> MGIISYVKKLFKRPAGEIMRMSSGNIGVYKLDDSRVDYELARELYQNKNANYKLGSSFVRPIVNSTTGFMGVPHFQIEDEEAQYILDEFVLDNTSKMLKTHTDSLKQGDCYIWITREERENPLYPDKKVRLIYNFISPEEVKEIILDPTTKEPIAYILESQNEWTDLGENKRKAKVKQIITAESRFVEVEGDKIEGLEEGETPNVWGFIPIIHFKNEADETLKYGQSDIEPIEPLLKAYHDVMLHALKGSKMHSTPKLKLKLTDVASFLAHNFGVEDPVKFAKEGGKINLDGHEILFLNKDEEAEFVEVKSAIGDAKELLKLLFYCIVDVSETPEFIFG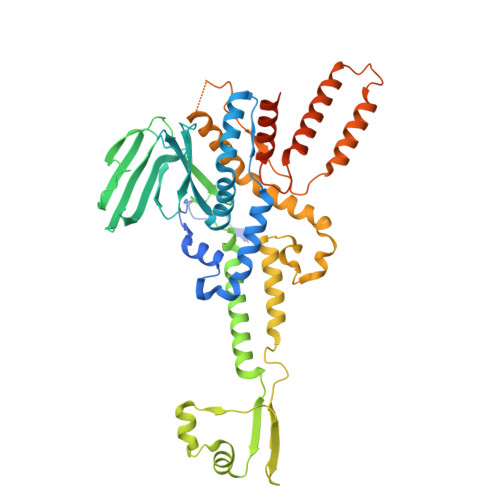VHTPSALASVKEQMPIMVNKIRRKREQFTNSWQLLARMVLIMSSNSSGMKYSSYDVTIGWDEVNPRDDKELAETLEKVCCALDKALEGGFISEESTVNFLAQYIDTMSNYISDDPEREGEREKIIKTKMLKYRLDDSQGLNDESNEIEKEINKIKDNNGNG> MSALSLLILGLLTAVPPASCQQGLGNLQPWMQGLI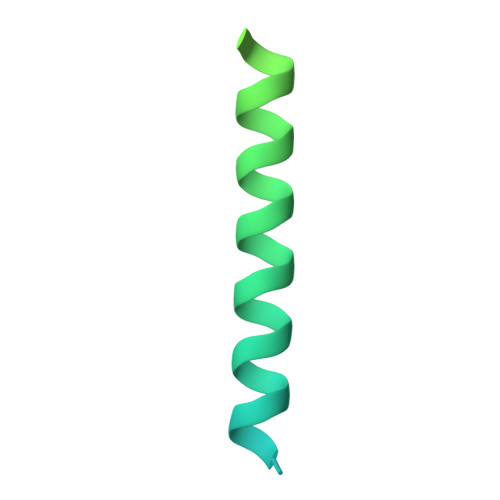AVAVFLVLVAIAFAVNHFWCQEEPEPAHMILTVGNKADGVLVGTDGRYSSMAASFRSSEHENAYENVPEEEGKVRSTPM>[2x]IVGGYTCEENSLPYQVSLNSGSHFCGGSLISEQWVVSAAHCYKTRIQVRLGEHNIKVLEGNEQFINAAKIIRHPKYNRDTLDNDIMLIKLSSPAVINARVSTISLPTAPPAAGTECLISGWGNTLSFGADYPDELKCLDAPVLTQAECKASYPGKITNSMFCVGFLEGGKDSCQRDAGGPVVCNGQLQGVVSWGHGCAWKNRPGVYTKVYNYVDWIKDTIAANS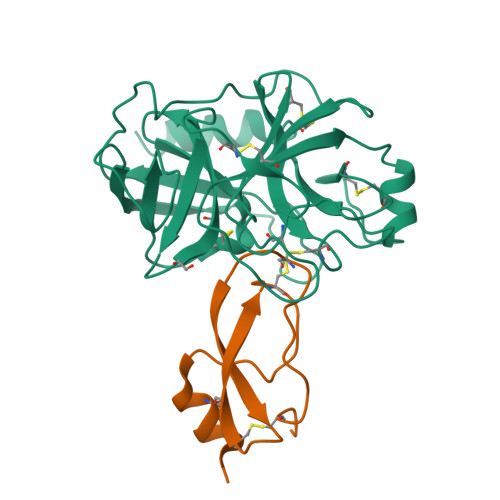;>YVDYKDDDDKEVEVCSEQAEVGPCRARFSRWYFDVTEGKCAPFVYGGCGGNRNNFDTEEYCMAVCGSAIPRHHHHHHAAAN[2x]> MSLTNDERILSWNETPSKPRYTPPPGAIDAHCHVFGPMAQFPFSPKAKYLPRDAGPDMLFALRDHLGFARNVIVQASCHGTDNA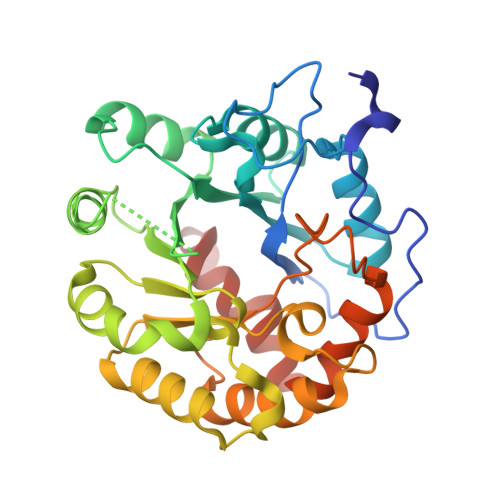ATLDAIARAQGKARGIAVVDPAIDEAELAALHEGGMRGIRFNFLKRLVDDAPKDKFLEVAGRLPAGWHVVIYFEADILEELRPFMDAIPVPIVIDHMGRPDVRQGPDGADMKAFRRLLDSREDIWFKATCPDRLDPAGPPWDDFARSVAPLVADYADRVIWGTNWPHPNMQDAIPDDGLVVDMIPRIAPTPELQHKMLVTNPMRLYWSEEMEGHHHHHH> MGAAVTLNRIKIAPGIADIRDKYMELGFNYPEYNRAVKFAEESYTYYYETSPGEIKPKFCLIDGMSIDHCSSFIVPEFAKQYVLIHGEPCSSFKFRPGSLIYYQNEVTPEYIKDLKHATDYIASGQRCHFIKKDYLLGDSDSVAKCCSKTNTKHCPKIFNNNYKTEHCDDFMTGFCRNDPGNPNCLEWLRAKRKPAMSTYSDICSKHMDARYCSEFIRIIRPDYFTFGDTALYVFCNDHKGNRNCWCANYPKSNSGDKYLGPRVCWLHECTDESRDRKWLYYNQDVQRTRCKYVGCTINVNSLALKNSQAELTSNCTRTTSAVGDVHPGEPVVKDK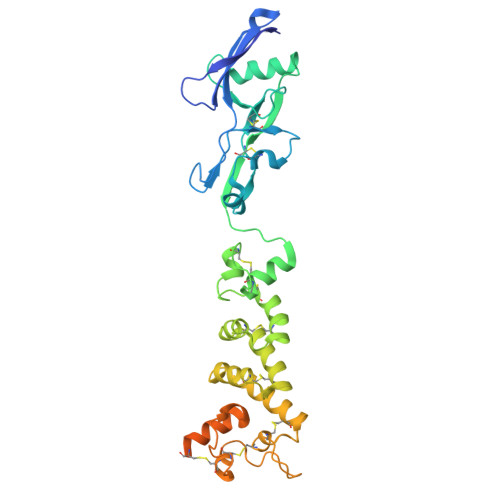IKLPTWHHHHHH>MTDTSSSSSSSSASSVSAHQPTQEKPAKTYDDAASESSDDDDIDALIEELQSNHGVDDEDSDNDGPVAAGEARPVPEEYLQTDPSYGLTSDEVLKRRKKYGLNQMADEKESLVVKFVMFFVGPIQFVMEAAAILAAGLSDWVDFGVICGLLMLNAGVGFVQEFQAGSIVDELKKTLANTAVVIRDGQLVEIPANEVVPGDILQLEDGTVIPTDGRIVTEDCFLQIDQSAITGESLAVDKHYGDQTFSSSTVKRGEGFMVVTATGDNTFVGRAAALVNKAAGGQGHFTEVLNGIGIILLVLVIATLLLVWTACFYRTNGIVRILRYTLGITIIGVPVGLPAVVTTTMAVGAAYLAKKQAIVQKLSAIESLAGVEILCSDKTGTLTKNKLSLHEPYTVEGVSPDDLMLTACLAASRKKKGLDAIDKAFLKSLKQYPKAKDALTKYKVLEFHPFDPVSKKVTAVVESPEGERIVCVKGAPLFVLKTVEEDHPIPEDVHENYENKVAELASRGFRALGVARKRGEGHWEILGVMPCMDPPRDDTAQTVSEARHLGLRVKMLTGDAVGIAKETCRQLGLGTNIYNAERLGLGGGGDMPGSELADFVENADGFAEVFPQHKYRVVEILQNRGYLVAMTGDGVNDAPSLKKADTGIAVEGATDAARSAADIVFLAPGLSAIIDALKTSRQIFHRMYSYVVYRIALSLHLEIFLGLWIAILDNSLDIDLIVFIAIFADVATLAIAYDNAPYSPKPVKWNLPRLWGMSIILGIVLAIGSWITLTTMFLPKGGIIQNFGAMNGIMFLQISLTENWLIFITRAAGPFWSSIPSWQLAGAVFAVDIIATMFTLFGWWSENWTDIVTVVRVWIWSIGIFCV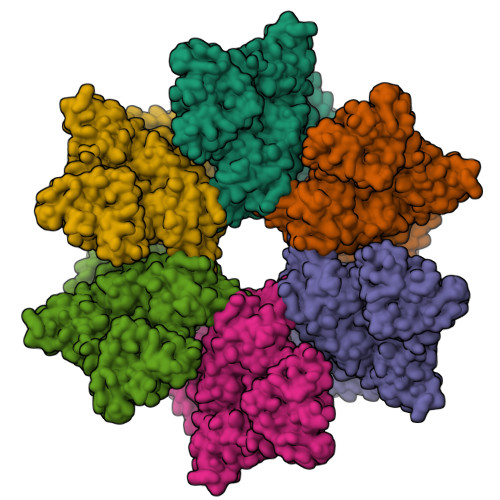LGGFYYEMSTSEAFDRLMNGKPMKEKKSTRSVEDFMAAMQRVSTQHEKET[6x]>[2x]SNAMNPLVIKLGGVLLDSEEALERLFTALVTYREKHERPLVIMHGGGCLVDELMKRLALPVVKKNGLRVTPADQIDIITGALAGTANKTLLAWAVKHQINAVGLCLADGNTVTVTLLDAELGHVGKAQPGSAALVQTLLAAGYMPIISSIGITVEGQLMNVNADQAATALAATLGADLI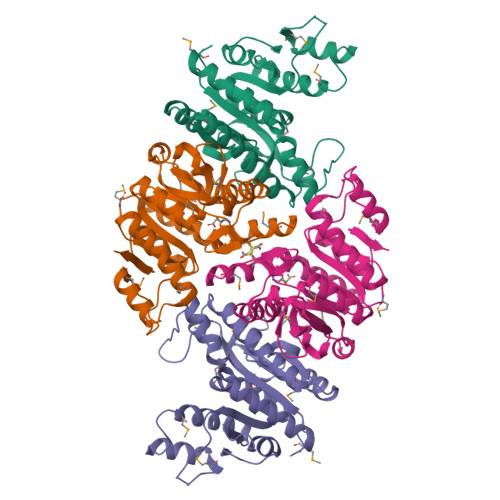LLSDVSGILDGKGQRIAEMTAQKAEQLIAQGIITDGMVVKVNAALDAARSLGRPVDIASWRHSEQLPALFNGVPIGTRISV>MAMITGGELVVRTLIKAGVEHLFGLHGAHIDTIFQACLDHDVPIIDTRHEAAAGHAAEGYARAGAKLGVALVTAGGGFTNAVTPIANAWLDRTPVLFLTGSGALRDDETNTLQAGIDQVAMAAPITKWAHRVMATEHIPRLVMQAIRAALSAPRGPVLLDLPWDILMNQIDEDSVIIPDLVLSAHGARPDPADLDQALALLRKAERPVIVLGSEASRTARKTALSAFVAATGVPVFADYEGLSMLSGLPDAMRGGLVQNLYSFAKADAAPDLVLMLGARFGLNTGHGSGQLIPHSAQVIQVDPDACELGRLQGIALGIVADVGGTIEALAQATAQDAAWPDRGDWCAKV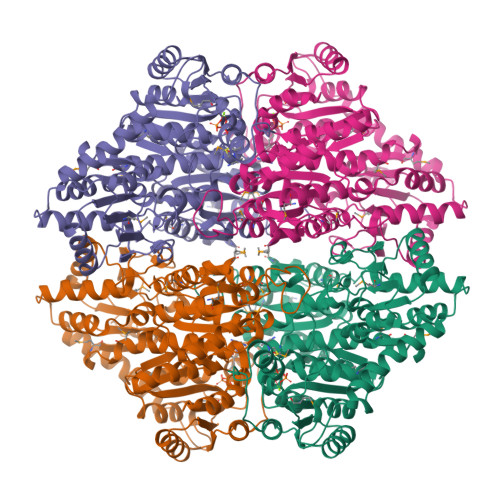TDLAQERYASIAAKSSSEHALHPFHASQVIAKHVDAGVTVVADGALTYLWLSEVMSRVKPGGFLCHGYLGSMGVGFGTALGAQVADLEAGRRTILVTGDGSVGYSIGEFDTLVRKQLPLIVIIMNNQSWGATLHFQQLAVGPNRVTGTRLENGSYHGVAAAFGADGYHVDSVESFSAALAQALAHNRPACINVAVALDPIPPEELILIGMDPFA[4x]>[2x]TPEMPVLENRAAQGNITAPGGARRLTGDQTAALRNSLSDKPAKNIILLIGDGMGDSEITAARNYAEGAGGFFKGIDALPLTGQYTHYALNKKTGKPDYVTDSAASATAWSTGVKTYNGALGVDIHEKDHPTILEMAKAAGLATGNVSTAELQH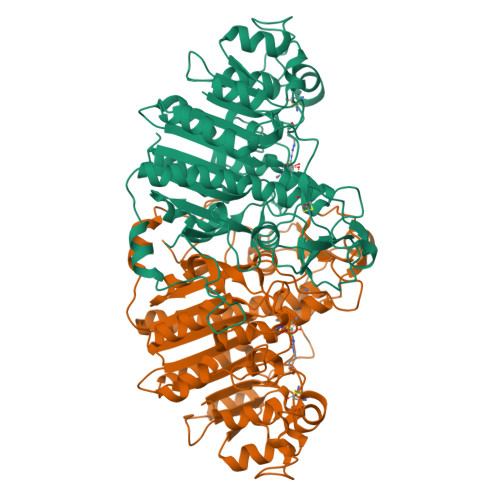ATPAALVAHVTSRKCYGPSATSQKCPGNALEKGGKGSITEQLLNARADVTLGGGAKTFAETATAGEWQGKTLREEAEARGYQLVSDAASLNSVTEANQQKPLLGLFADGNMPVRWLGPKATYHGNIDKPAVTCTPNPQRNDSVPTLAQMTDKAIELLSKNEKGFFLQVEGASIDKQNHAANPCGQIGETVDLDEAVQRALEFAKKEGNTLVIVTADHAHASQIVAPDTKAPGLTQALNTKDGAVMVMSYGNSEEDSQEHTGSQLRIAAYGPHAANVVGLTDQTDLFYTMKAALGLK>MTAPTVPVALVTGAAKRLGSGIAEGLHAEGYAVCLHYHRSAAEANTLAATLNARRPNSAIPVQADLSNVAKAPAGGADGAAPVTLFKRCADLVAACYTHWGRCDVLVNNASSFYPTPLLRKDEDGHVPCVGDREAMEAAAADLFGSNAMAPYFLIKAFAHRVADTPAEQRGTNYSIVNMVDAMTSQPLLGYTIYTMAKGALEGLTRSAALELAPLQIRVNGVGPGLSVLADDMPPAVREDYRSKVPLYQRDSSAAEVSDVVIFLCSSKAKYVTGTCVKVDGGYSLTRA[2x]

A promising target with respect to infection with Leishmania sp. is the NADPH-dependent short-chain dehydrogenase/reductase pteridine reductase (PTR1; EC 1.5.1.33). This enzyme is unique to trypanosomatid parasites, where it supports the provision of reduced biopterins that are necessary for meta­cyclogenesis and which are implicated in resistance to reactive oxygen and nitrogen species in Leishmania. PTR1 catalyzes the reduction of biopterin to 7,8-dihydrobiopterin as well as its subsequent reduction to 5,6,7,8-tetrahydrobiopterin. PTR1 displays a sequential ordered mechanism, with first cofactor binding and then substrate; following reduction the product leaves, followed by oxidized cofactor.

The structure of apo LdPTR1 has been solved to 2.5 Å resolution. Ammonium sulfate was the precipitant for crystal growth and a sulfate ion binds in a polar cavity formed by the β1–α1 turn and the loop between β2 and α2, accepting hydrogen bonds donated from three main-chain amides (His38, Arg39 and Ser40) and Ser40 OG. This polar cavity is the binding site for the adenine 2′-­phosphate group of the cofactor. Since sulfate binding blocks the 2′-­phosphate-binding site, NADP+ is not present and this leads to disorder in the substrate-binding part of the active site. However, the residues near the catalytic site were poorly ordered in contrast to the same regions of LmPTR1 and TbPTR1, with no electron density corresponding to NADP+ or methotrexate, ligands that were present in the crystallization conditions in a fivefold molar excess. Missing segments include residues 70–80 (the loop linking β3 and α3), 112–132 (the β4–α4 loop) and 227–254 (the β6–α6 loop). However, the β4–α4 loop is well ordered in LmPTR1 but is missing in LdPTR1. This means that in LdPTR1, Phe113, which is a critical residue, is disordered. The absence of the β4–α4 loop vacates an area in the active-site cleft, allowing the β5–α5 loop of LdPTR1 to adopt a different position to fill the gap. We conclude that owing to the disorder this crystal form is not suitable for characterizing the interactions of LdPTR1 with inhibitors.> MHAALTPLTNKYRFIDVQPLTGVLGAEITGVDLREPLDDSTWNEILDAFHTYQVIYFPGQAITNEQHIAFSRRFGPVDPVPILKSIEGYPEVQMIRR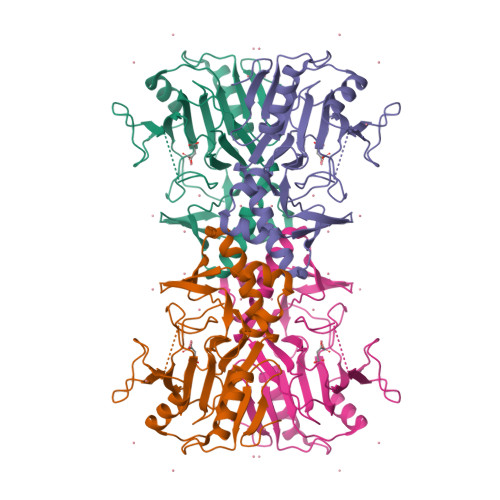EANESSRFIGDDWHTDSTFLDAPPAAVVMRAIEVPEYGGDTGFLSMYSAWETLSPTMQATIEGLNVVHSATKVFGSLYQATNWRFSNTSVKVMDVDAGDRETVHPLVVTHPVTGRRALYCNQVYCQKIQGMTDAESKSLLQFLYEHATKFDFTCRVRWKKDQVLVWDNLCTMHRAVPDYAGKFRYLTRTTVAGDKPSR Mitochondrial ATP synthase consists of the soluble F1 and membrane-bound Fo subcomplexes and occurs in dimers that assemble into oligomers to induce the formation of inner-membrane folds, called cristae. Dissociation of ATP synthase dimers into monomers results in the loss of native cristae architecture and impairs mitochondrial function. Here, we report cryo-EM structures of the intact ATP synthase dimer from Trypanosoma brucei in ten different rotational states. Although overall dimer architecture varies among eukaryotes, we find that subunit-g together with subunit-e form an ancestral oligomerization motif, which is shared between the trypanosomal and mammalian lineages.

Finally, particles with both monomers in rotational state 1 were selected, and the consensus structure of the dimer was refined to 3.2 Å resolution. Unlike the wide-angle architecture of dimers found in animals and fungi, the T. brucei ATP synthase displays an angle of 60° between the two F1/c-ring subcomplexes. Despite sharing a set of conserved Fo subunits, the T. brucei ATP synthase dimer displays a markedly different dimer architecture compared to previously determined structures. Second, unlike mammalian and fungal ATP synthase, in which the peripheral stalks extend in the plane defined by the two rotary axes, in our structure the monomers are rotated such that the peripheral stalks are offset laterally on the opposite sides of the plane. Due to the rotated monomers, this architecture is associated with a specific dimerization interface, where two subunit-g copies interact homotypically on the C2 symmetry axis. Both copies of H1-2g extend horizontally along the matrix side of the membrane, clamping against each other. Thus, the ATP synthase dimer is assembled via the subunit-e/g module.

>MFLFFFCDLFWLRLLLCMYYCVWSRLCFIVYFNCLMLIFDFLLFCLFDLYLFVGLCLFLLLWFMLFNLYSLILYYCITYLNLYLLFCIVFLLYIAFLFLFCFLCDFFLFNNLLVGDSFMDVFFIRFLLCFLECFSLLCRCLSTFLRLFCNLLSSHFLLLMFFDFFYFIFVFFFYGVFCYWFILFIFVFCFCLLFYVFLYLLDLFAAILQLFIFCNMILQLIMDFLLFLLFV[2x];>[6x]MRRFGSKFASGLASRCALACPLASAATAPAGASTTSSTSSAQKSFFKTTEMIGYVHSIDGTIATLIPAPGNPGVAYNTIIQIQVSPTTFAAGLVFNLEKDGRIGIILMDNITEVQSGQKVMATGQLLHIPVGAGVLGKVVNPLGHEVPVGLVTRSRRLLDSTLGKVDTGAPNIVSRSPVNYNLLTGFKAVDTMIPIGRGQRELIVGDRQTGKTSIAVSTIINQVRINQQILSKNAVISIYVSIGQRCSNVARIHRLLQSYGALRYTTVMAATAAEPAGLQYLAPYAGVTMGEYFMNRGRHCLCVYDDLSKQAVAYRQISLLLRRPPGREAYPGDVFYLHSRLLERAAMLSPGKGGGSVTALPIVETLSNDVTAYIVTNVISITDGQIYLDTKLFTGGQRPAVNIGLSVSRVGSSAQNAAMKGVAGKLKGILAEYRKLAADSVGGQQVQTIPMIRGARFVALFNQKQPSYFMNAIVSLYACLNGYLDDVKVQYVKFYEYLLVHRDLGIMYGTAKNKFFYMYVQELNYLIRFFTLNSPILHGELEEMLKQHTHLFLQHYQSKMNAIKSEKDVKALKNLLYSCKRAV;>[2x]MLRRLGANVSNMARPMNKYAVTVSPRRHLEPMSTWYLASWAMVWYYAFFFWMPMVWTDIMVPSFVYNKLPVIHFLQEKRAEQKLRRVLDETYTEWTEELDQAHVTDAITRSLNI;>MRRVSSPNITIQSVRWISGVSPLLYFPPTTTSTTNREDQINKNTNIAIQMIKRYKGEVPPHYTRKSSATIEQVEKEIDALLGGAEKLRKTSTDDQPMDKLTLMERCLRHALWSYHKEEGRYDFDQIGRWVVYTPEDEVKLAQLKREVEAKEKLAALRKRREEEGLPGGPVPRINWPQEYSSFIDREPVVAKRIRYDTLASTTLERDEKQIESTLQQYRRASQDKRLDDLVDLLERFKPVLAREAIMQRLTIKHLEGQLGVWRYMDWCPEVRDRAELEVDITGWQWWSPLEERRLLPVRLRSVNEVREIMSKTQAKKSAEAAERNPIVTQTSTGDNARDRLLKEVLALQARINQRDEVEPSQTEQKKKAHH[2x];>[6x]MLTRFRSAVLRGAVSITGARAASTAPVADHKGRVGHVSQVIGAVVDVHFADGVPPVLTALDVVDKLGRDEPLTLEIVQHLDAHTGRCIAMQTTDLLKLKAKVVSTGGNISVPVGRETLGRIFNVLGDAIDQRGPVGEKLRMPIHAVAPKLADQAAEDAVLTTGIKVIDLILPYCKGGKIGLFGGAGVGKTVIIMELINNVAKGHGGFSVFAGVGERTREGTDLYLEMMQSKVIDLKGESKCVLVYGQMNEPPGARARVAQSALTMAEYFRDVEGQDVLLFIDNIFRFTQANSEVSALLGRIPAAVGYQPTLAEDLGQLQERITSTTKGSITSVQAVYVPADDITDPAPATTFSHLDATTVLDRAVAESGIYPAVNPLECASRIMDPDVISVDHYNVAQDVVQMLTKYRELQDIIAVLGIDELSEEDKLIVDRARKLVKFLSQPFQVAEVFTGMTGHYVQLDDTIDSFSGLLMGTYDQVPEMAFYMVGGINSVLEKAKKMAEEAAELEKMRRARVAQASS;>MQGSWSVLKKNCSNFFPGLLAFAQQTQEAYGIWLRIYNRQQKYGPTDFVEQSETFSPDYHKRFHSQDKNMWVDKELCTEVSQKEVARLMTYKLDMWRMAHCAGALLATGGYAIPFGLFWLANDTWVPSSFNLTGEELRAWREAQDLYRYRSAPSYLTDTKWHFDFHAYPWNETQERAWDDLFEKNDVRRDPKVVRPAAEMYDGFIKFELIRRKSLRHLCRSMNIPTFPMLARLCNGTRVRDYWNLAWCEDYMVITQRLHESMTDEELYDYAWRRYLAPYDKNLNREQLMERVEDYFEFLGPDFVAHGKAPNLVILTNYVLGYYNDPAYLEGDISELDKNDYDHLASWGKDAFLRRLEFENGPLRDQVEAHTQRLLAERAAIAKGDNAAAVEGRHTA[2x];>[2x]MVLFSTYRSSRLVSKEFLHGPVMRFRALGEYYFQRAWNGTLNWALPGEYRLYAVMIPFIYFYHRWHNDHTLDRDHVEKAMIMRWGGTLEDVRKLSAKDQLRVRCFTDIEKLYSAYGPKDTYLQPPGDTLPGKDFYRKAGGAQAHH;>[2x]MSKQLTFISAGATAAVLQSASAIVSKVAGGRVQTKTAKEAGRHAVVVGPETPIGVHTAVTEVPKSAQDPLFSGVSTVVVRAVLPRAAPDSVQLRDALDVYASAGIDTKEEVRSATEAFKKSAEVAVGKAKAKGVKRIVLVVKQASKHNCINELFKKISTETIESAGLTTEVVGTAAVANQLIVNPESLGVVLLNDVAATEQIELAFAGVVGGVSRVYHTVEGGKISAGHSFKSVALAVAQELRELGLSSEADKVEAAASKNPRAVVSAL;>MSGKLRLYKEKLEGYNRFYSIVKTIKMVTLAKYRAAQGRIRTRDFSLRYTELAFSKPQASRDAVVAAKNALVYIPITTNRGSCGALNSNIVRCIDSVVSSKMVLMPVGKRGIDSFSKLYPDEFRYGIINDMKESMHFGYATFVIENAYEVSKDADRYQVIFNRFVSAGVQRNAVYNIPSYEKWKEDLADAASSDNQKNRYLFANALQNEEEQLIRDFFDFHAALAVLNAVGENELSEQAARLVAVEGQLTNISSLQQRTSSLYNKTRQFGITAALIEILSAMSSLEGNAMKGVRRNKFWEGAVTK[2x];>[2x]MRRTFISFSAASAAAAAPVTSTKMQTLHKLLTGEVSFKNKAPVKDCNIVHQFGENWATELSAYAKTLPAEQQKIIVRQIARVKLTRYTVAELAAYCGDGPALLDETARAANIEQGVAFVKAKGVEAFEKYVAEESTNANWKPEEAKKFIEDVKAKAK;>[2x]MFRTFGRRLVSCTLPLLQSAPHDLPEGFEFMEHKVVNKDIHAPHENLETLRLTLTRQDEFLLREEPVKCVTVTGTNGEYGIYPGHAYKIVQLNPSPLTVEYTDGTTKKYFVSGGFAHINNEGSCDVNTVECTLLDDLDLAIAEKELAAQQAALGSAKDDKAKSVVEIRISVIEAVIAALKHH;>MVYTRWKCDRLPVFQLKLFTQEYPMHAAVGIFTIIFLWKHMSHCSEETERKYGWWAGYPYWRDPIARRNETKYKQMIINNDVDITHPKWTGCSVEQLEELSRVV[2x];>MIRRSCALLSSSWRDHGISYLKYLNVCTETLHSTVKESRRAKYERWSKPCYTAQRPDGAGGQETIDKVPIHTKDY[2x];>[2x]MTKYELKMQYFDEWMIRWRKFQTESDWEIEKGRQWWRRFNMAVSGALFCGLVLYTSGTATLKRQYGLPHFFDIGVDGQAKETMLKTLTSRWRYTPQGYGRVLITGVPTYILFVTLEHYRERRRMQQYLQQNTVFGEQMRRLLSTGKIEEYLPVNIKATLPASQQAIYNY;>[6x]MMRRVYSPVFCSVAAARFAATSAAKKYDLFGYEVDTNTAPWIEKIKKCKYYDEAGEVLVNMNVSNCPPDIATYNATLQCIYQSPSKQSTPVDNESKFCAMMDLLEEMQHRNRLKPNEESWTWVMKECVKSGQFRLGYCIQQVMETECKGCPADLVKANEANAQKAKTEGKEHPGHLSQQAGLFDVKVE;>[2x]MLRRSSAALIRRTPVRHSGGELFVRPKLEEIPPADQCRGFFGPLNDSLKFLRLLDIKWMMNRAVAMRREYLIATPTLFTFIWMFTWKGAVIYFWGDRAPPRRMDWNTEETGRLPLGFKPTPAPL;>[2x]MSAKAAPKTLHQVRNVAYFFAAWLGVQKGYIEKSANDRLWVEHQRKVRQQNVERQQALDSIKLMQQGVRATTPGQLEGVPAELQQLAEAFTK;>[2x]MSSTKCAVACKIMTPLCNAASKVQARSAKKLAALTDAGIQKTISEHNANGTDAAVSSTKRYLAEQRQLFHYRVVRFFDECHYIISGEYFAQYTKVNLIWDLRFLTKLVVLFLIGTVLGRQSIFPPIDPDSPLVEALVTKVNPNY;>[2x]MFRRLSSSARAVVAARFYTPPEGLKKLYASDFENSKYPLNIVPSDSVLFAKFLYKAAEEKGNFDNILSDFQKIAAAASKLPIFWERTAVVEKIPEFKQLSEPTFFTLVWMQNNGMLELIQEVAEVYETFVNAKQKKAVAKIFVAPGGEKNVEEARRVAEELHKGLKELADYTLVLKTVVDRTIVKGFAVELAGQYVNKAEGQQKQAGRADEVDYTNLPAPKPQKTVWDDNIETEVLRKYLDGLSQYDMEEAKYGV;>[2x]MLRKTPLFAMATTRKALVGNGPTFSTGGECMNTCDIQNAFPMNDRGVRSSSPFQEPNTAIYDSYLAWTYFQPMDVHIEKLPAPEAKYYQRHTKKPWDVSSTELTEIQSRKKYFQTLGYLVAFIYLYFLMPKEKSFSGLSGPDGHWIMLPKGRPELF;>MSSGFHFHDVSNDAIKGMPPSEALHKHLENAQLAHRICLAKALKAGEPPVEKCALTWGEVLIRYQAWSEYRPPFQDSVAQAKYKKYWSKKRQEEDDKNPFK[2x];>[20x]MMRRLALQSSIRRATPFATPLVASTKALNPMCSAITIREASTVAISVQGLHYVGTGLAAIALAGVGLGIGTIFGNLLVACARQPNLTKMLFNYAILGFALTEAIGLFALMLAFLMLFS;>[2x]MLRRLVPRVMMAPMGGATALCTSRGYNMLVFRDPKRRPQLSEEERAKVVVNQAEWPEEFKDFDPDDPYKNSPEIIKGMSSWNLFLWGVECAFIYQFYELVFPKSI;>[2x]MTENIEAVMSDFWSNPADHFRPNLKALTLYAERQHYVDRWLHVKERWLAPWYLPWWSPLFQLGTWYSQRSRNLFLVENHLSYRPYKFRRNDEDRNNPY;>MLLGGFVPRRFSQFNRDPCWMFFIFSVGFWLGEYPAMMIKYNARDLVYDPHRYVWSHHDDHH[2x]>MGSSHHHHHHSQDPNSASLPGIDEHTTSEELITGDNEWHKLVIPKGSDWQIDLKAEGKLIVKVNSGIVEIFGTELAVDD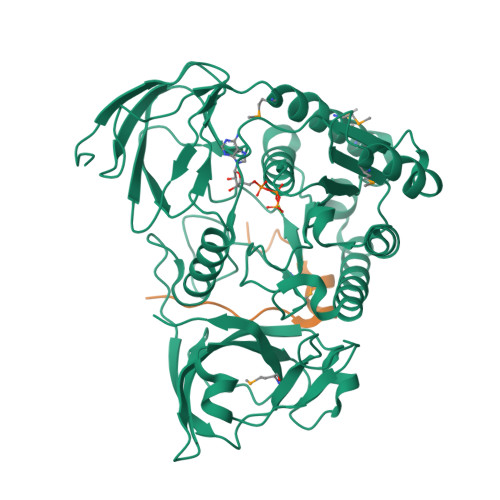EYTFQNWKFPIYAVEETELLWKCPDLTTNTITVKPNHTMKYIYNLHFMLEKIRMSNFEGPRVVIVGGSQTGKTSLSRTLCSYALKFNAYQPLYINLDPQQPIFTVPGCISATPISDILDAQLPTWGQSLTSGATLLHNKQPMVKNFGLERINENKDLYLECISQLGQVVGQRLHLDPQVRRSGCIVDTPSISQLDENLAELHHIIEKLNVNIMLVLCSETDPLWEKVKKTFGPELGNNNIFFIPKLDGVSAVDDVYKRSLQRTSIREYFYGSLDTALSPYAIGVDYEDLTIWKPSNVFDNEVGRVELFPVTITPSNLQHAIIAITFAERRADQATVIKSPILGFALITEVNEKRRKLRVLLPVPGRLPSKAMILTSYRYLE[2x];>[2x]GSQNTANTGISNSNLNTTTTRKNIQSRNWYLSDSQWAAFKDDEITSTKHKNDYTDPHANKNIDKSALNIHADENDEGSVDNTLGSDRSNELEIRGKYVVVPETSQDMAFK6-benzyl-3-[3-(benzyloxy)phenyl]-4,6-dihydropyrido[4,3-d]pyrimidine-2,7(1H,3H)-dione | C27 H23 N3 O3 | 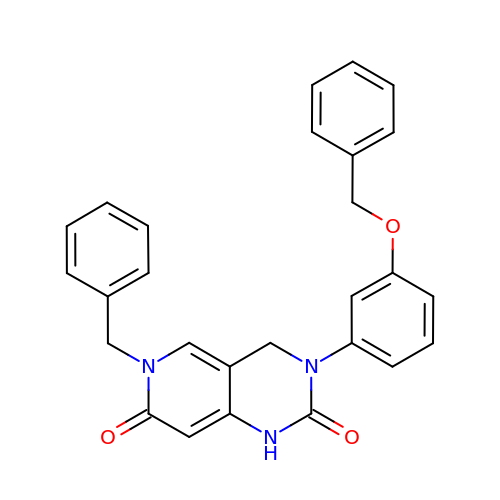BHMKGMWMMMZMJN-UHFFFAOYSA-N>[2x]GHMVSCSAPGKIYLFGEHAVVYGETAIACAVELRTRVRAELNDSITIQSQIGRTGLDFEKHPYVSAVIEKMRKSIPINGVFLTVDSDIPVGSGLGSSAAVTIASIGALNELFG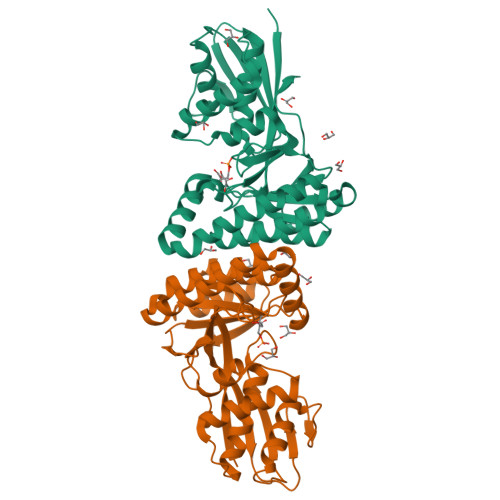FGLSLQEIAKLGHEIEIKVQGAASPTDTYVSTFGGVVTIPERRKLKTPDCGIVIGDTGVFSSTKELVANVRQLRESYPDLIEPLMTSIGKISRIGEQLVLSGDYASIGRLMNVNQGLLDALGVNILELSQLIYSARAAGAFGAKITGAGGGGCMVALTAPEKCNQVAEAVAGAGGKVTITKPTEQGLKVD> GPPVVEEDDVVGFDDEAQTVIDRLLEGSGDLEVIPVVGMPGLGKTTLATKIFKHPKIEYEFFTRLWLYVSQSYKTRELYLNIISKFTGNTKHCRDMSEKDLALKVQEILEEGGKYLIVLDDVWSTDAWDRIKIAFPKNDKGNRVLLTTRDHRVARYCNRSPHDL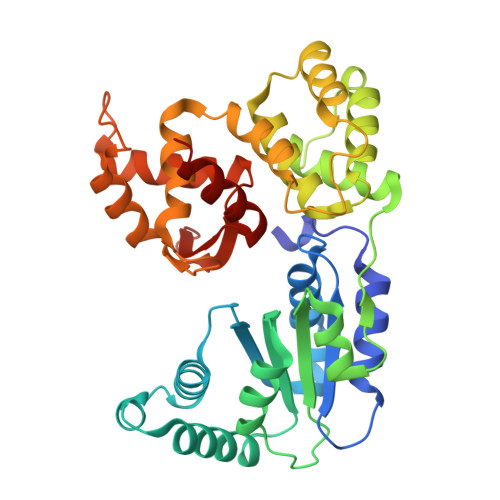KFLTDEESWILLEKRAFHKAKCLPELETNGKSIARKCKGLPLAIVVIAGALIGKSKTIKEWEQVDQSVGEHFINRDQPNSCDKLVRMSYDVLPYDWKACFLYFGTFPRGYLIPARKLIRLWIAEGFIQYRGDLSPECKAEEYLNELVNRNLVMVMQRTVDGQIKTCRVHDMLYEFCWQEATTE> MSHQKIIQDLIAWIDEHIDQPLNIDVVAKKSGYSKWYLQRMFRTVTHQTLGDYIR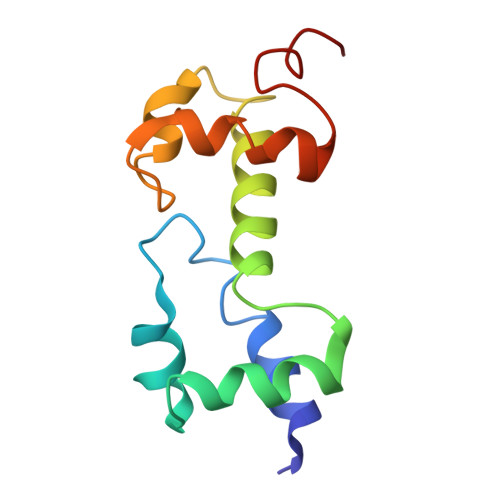QRRLLLAAVELRTTERPIFDIAMDLGYVSQQTFSRVFRRQFDRTPSDYRHRL>DTEKLIREKDEELRRMQEMLEKMQAQMQQS[4x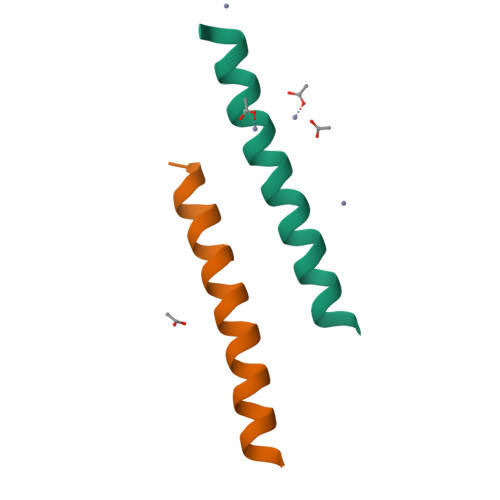]> PSAEECGYSDRVRSLTLGNSTITTQESANVVVGYGRWPEYLRDDEATAEDQPTQPDVATCRFYTLESVQWEKNSAGWWWKFPEALKDMGLFGQNMLYHYLGRAGYTIHVQCNASKFHQGCLLVVCVPEAEM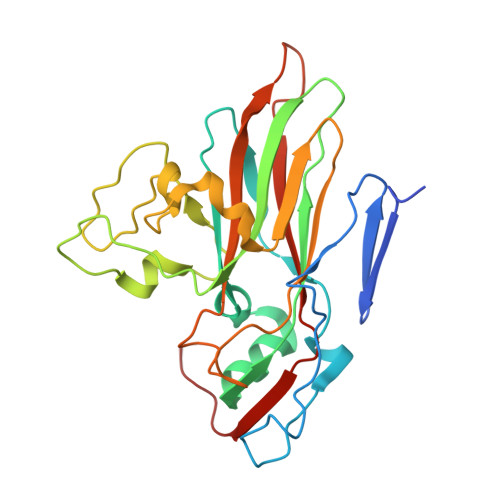GCSQTDKEVAAMNLTKGEAAHKFEPTKTNGEHTVQSIVCNAGMGVGVGNLTIYPHQWINLRTNNCATIVMPYVNSVPMDNMFRHYNFTLMVIPFAPLDYAAQASEYVPVTVTIAPMCAEYNGLRLAYQQ> GGGRMATTTAGLTDLKFRVVREDFADAVAWVARSLPTRPTIPVLAGVLLTGTDEGLTISGFDYEVSAEVKVSAEI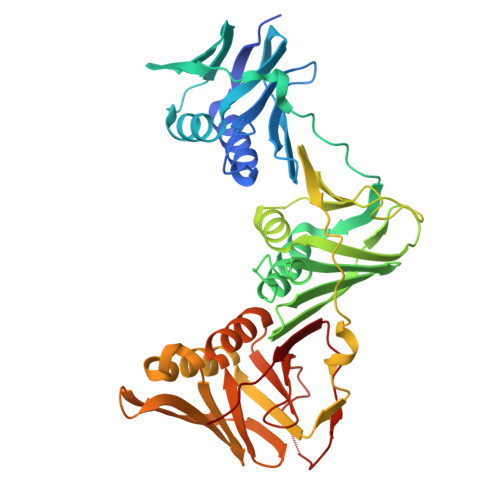ASAGSVLVSGRLLSDITKALPAKPVEVSVEGTRVSLTCGSARFSLPTLAVEDYPALPALPEETGVIASDLFAEAIGQVAVAAGRDDTLPMLTGIRVEISGESVVLAATDRFRLAVRELTWVTTAGDVEAAVLVPAKTLAEAAKAGTDGNQVHLALGSGASVGKDGLLGIRSEGKRSTTRLLDAEFPKFRQLLPAEHTAVATIGVAELTEAIKRVALVADRGAQIRMEFSDDTLKLSAGADDVGRAEEDLPVDFAGEPLTIAFNPTYLTDGLGSLHSERVTFGFTTPSRPAVLRPAGEDDGANGGSGPFPAAKTDYVYLLMPVRLPG To understand the mechanism in detail we determined the structure of CitS from the human pathogen Salmonella enterica by single-wavelength anomalous dispersion with crystals of seleno-methionine derivatized protein. In membrane vesicles and proteoliposomes, CitS from Klebsiella pneumoniae (KpCitS) was previously shown to transport citrate as HCit2- in a sodium-dependent manner. We observed similar transport properties for CitS from Salmonella enterica (SeCitS), which is closely related to KpCitS. Sodium transport is cooperative with a Hill coefficient of 1.89, whereas citrate is not, suggesting that citrate transport is coupled to at least two Na+ ions.

The asymmetric unit contains two homodimers of two protomers in different conformations. Each protomer has 13 helix elements (H1–H13), including eleven transmembrane helices (TMH) and two helix hairpins (H6, H12), with the N-terminus on the cytoplasmic side and the C-terminus on the outside. Helices H2-–7 and H8–13 are organized in two repeats with inverted topology, connected by a flexible cytoplasmic loop. Together, helices H5–7 of repeat 1 and H11–13 of repeat 2 form a bundle on either side of the central contact domains, which hold the dimer together through extensive hydrophobic interactions of H2, 4, 8 and 10. The two dimers in the asymmetric unit are similar, with an overall rmsd of 0.5 Å, whereas the protomers within one dimer differ substantially by an rmsd of 8.4 Å. Evidently, the whole bundle moves as a rigid body from its position in protomer A to that in protomer B, while the central dimer contact domain remains static. We conclude that protomer A is outward-facing and that protomer B faces inward. All four protomers show clear electron density for citrate in the binding site. In the outward-facing protomers, the citrate is closely coordinated by two arginines (Arg402, Arg428), two polar sidechains (Asn186, Ser405) and the protein backbone of both hairpins. In both outward-facing protomers, two Na+ ions are clearly resolved next to the citrate. In the case of SeCitS, comparison of the inward-facing protomers B and B’ indicates unambiguously that citrate is released before Na+, and that Na2 is released before Na1.

>MTNMTQASATERKGASDLLRFKIFGMPLPLYAFALITLLLSHFYNAIPTDLVGGFALMFVMGAIFGEIGKRLPIFNKYIGGAPVMIFLVAAYFVYAGIFTQKEIDAISNVMDKSNFLNLFIAVLITGAILSVNRKLLLKSLLGYIPTILAGIVGASLFGIVIGLCFGIPVDRIMMLYVLPIMGGGNGAGAVPLSEIYHSVTGRSREEYYSTAIAILTIANIFAIIFAALLDMVGKKYTWLSGEGELVRKASFKTEDDEKAGQITHRETAVGMVLSTTCFLLAYVVAKKILPSIGGVSIHYFAWMVLIVAALNASGLCSPEIKAGAKRLSDFFSKQLLWVLMVGVGVCYTDLQEIIDALTFANVVIAAIIVVGAVVGAAIGGWLIGFYPIESSITAGLCMANRGGSGDLEVLSACNRMNLISYAQISSRLGGGIVLVIASIVFSMMVLE[4x]Human protein E6AP/UBE3A, the founding member of the HECT-type ubiquitin ligase family, was originally identified as an associated partner of the viral oncoprotein E6 of human papillomaviruses (HPVs). The E6 oncoprotein from high-risk HPV types hijacks the ligase activity of the host E6AP to ubiquitinate the tumor suppressor p5313, leading to the aberrant p53 degradation. The HECT-type E3 ligases have a characteristic C-terminal HECT domain consisting of an N-lobe and a C-lobe that are responsible for E2 binding and ubiquitin acceptance, respectively. Here, by using cryogenic electronic microscopy, we reveal that the structures of full-length E6AP and E6AP/E6 complex are monomer and dimer of E6AP/E6 protomer, respectively.

After several rounds of 3D classification, we identified five distinct conformational states of the E6AP/E6 complex and resolved the structures of these five conformations at resolutions ranging from 2.6 to 4.4 Å. We therefore assigned the five conformations into one of two classes: attached (Att) or detached (Det). In all three Att conformations, the catalytic C-lobe of E6AP attaches to E6, whereas, in the two Det conformations, there are no interactions between the C-lobe and E6. We hereafter refer to the three Att conformations as Att1, Att2 and Att3 based on the distance between the tips of the two towers in a descending sequence: 74 Å in Att1, 71 Å in Att2, and 66 Å in Att3. (1) the two towers tilt towards each other around a region of intersect between the two α1-helices. As such, the conformation of E6AP/E6 complex changes from Att1, through Att2 to Att3. (2) When the two towers leant beyond a threshold, the Att conformation changed into a Det conformation. While the distance between the two towers varies among the three Att conformations, there is no detectable difference in the distance between the C-lobe and the inter-protomer E6. As the two towers underwent an outwards rotation, the Det2 conformation transformed into the Det1 conformation. Intriguingly, despite substantial variation in the structure of the E6AP/E6 complex, the inter–α1-helical interaction remains intact; albeit there are some changes at the interface between the two α1-helices (238 Å2 for Att1, 222 Å2 for Att2, 209 Å2 for Att3, 157 Å2 for Det1 and 145 Å2 for Det2). The Det and Att conformations of the E6AP/E6 complex presented in this study should be structurally relevant to these accepting and donating processes, respectively.

>[2x]MEKLHQCYWKSGEPQSDDIEASRMKRAAAKHLIERYYHQLTEGCGNEACTNEFCASCPTFLRMDNNAAAIKALELYKINAKLCDPHPSKKGASSAYLENSKGAPNNSCSEIKMNKKGARIDFKDVTYLTEEKVYEILELCREREDYSPLIRVIGRVFSSAEALVQSFRKVKQHTKEELKSLQAKDEDKDEDEKEKAACSAAAMEEDSEASSSRIGDSSQGDNNLQKLGPDDVSVDIDAIRRVYTRLLSNEKIETAFLNALVYLSPNVECDLTYHNVYSRDPNYLNLFIIVMENRNLHSPEYLEMALPLFCKAMSKLPLAAQGKLIRLWSKYNADQIRRMMETFQQLITYKVISNEFNSRNLVNDDDAIVAASKCLKMVYYANVVGGEVDTNHNEEDDEEPIPESSELTLQELLGEERRNKKGPRVDPLETELGVKTLDCRKPLIPFEEFINEPLNEVLEMDKDYTFFKVETENKFSFMTCPFILNAVTKNLGLYYDNRIRMYSERRITVLYSLVQGQQLNPYLRLKVRRDHIIDDALVRLEMIAMENPADLKKQLYVEFEGEQGVDEGGVSKEFFQLVVEEIFNPDIGMFTYDESTKLFWFNPSSFETEGQFTLIGIVLGLAIYNNCILDVHFPMVVYRKLMGKKGTFRDLGDSHPVLYQSLKDLLEYEGNVEDDMMITFQISQTDLFGNPMMYDLKENGDKIPITNENRKEFVNLYSDYILNKSVEKQFKAFRRGFHMVTNESPLKYLFRPEEIELLICGSRNLDFQALEETTEYDGGYTRDSVLIREFWEIVHSFTDEQKRLFLQFTTGTDRAPVGGLGKLKMIIAKNGPDTERLPTSHTAFNVLLLPEYSSKEKLKERLLKAITYAKGFGML;>[2x]FQDPQERPRKLPQLCTELQTTIHDIILECVYCKQQLLRREVYDFAFRDLCIVYRDGNPYAVCDKCLKFYSKISEYRHYSYSLYGTTLEQQYNKPLSDLLIRCINCQKPLSPEEKQRHLDKKQRFHNIRGRWTGRCMSCSRS> MPYSVGFREADAATSFLRAARSGNLDKALDHLRNGVDINTCNQNGLNGLHLASKEGHVKMVVELLHKEIILETTTKKGNTALHIAALAGQDEVVRELVNYGANVNAQSQKGFTPLYMAAQENHLEVVKFLLENGANQNVATEDGFTPLAVALQQGHENVVAHLINYGTKGKVRLPALHIAARNDDTRTAAVLLQNDPNPDV;> MSSKYPRSVRRCLPLWALTLEAALILLFYFFTHYDASLEDQKGLVASYQVGQDLTVMAALGLGFLTSNFRRHSWSSVAFNLFMLALGVQWAILLDGFLSQFPPGKVVITLFSIRLATMSAMSVLISAGAVLGKVNLAQLVVMVLVEVTALGTLRMVISNIFNTDYHMNLRHFYVFAAYFGLTVAWCLPKPLPKGTEDNDQRATIPSLSAMLGALFLWMFWPSVNSPLLRSPIQRKNAMFNTYYALAVSVVTAISGSSLAHPQRKISMTYVHSAVLAGGVAVGTSCHLIPSPWLAMVLGLVAGLISIGGAKCLPVCCNRVLGIHHISVMHSIFSLLGLLGEITYIVLLVLHTVWNGNGMIGFQVLLSIGELSLAIVIALTSGLLTGLLLNLKIWKAPHVAKYFDDQVFWKFPHLAVGF;>[2x]MRFTFPLMAIVLEIAMIVLFGLFVEYETDQTVLEQLNITKPTDMGIFFELYPLFQDVHVMIFVGFGFLMTFLKKYGFSSVGINLLVAALGLQWGTIVQGILQSQGQKFNIGIKNMINADFSAATVLISFGAVLGKTSPTQMLIMTILEIVFFAHNEYLVSEIFKASDIGASMTIHAFGAYFGLAVAGILYRSGLRKGHENEESAYYSDLFAMIGTLFLWMFWPSFNSAIAEPGDKQCRAIVNTYFSLAACVLTAFAFSSLVEHRGKLNMVHIQNATLAGGVAVGTCADMAIHPFGSMIIGSIAGMVSVLGYKFLTPLFTTKLRIHDTCGVHNLHGLPGVVGGLAGIVAVAMGASNTSMAMQAAALGSSIGTAVVGGLMTGLILKLPLW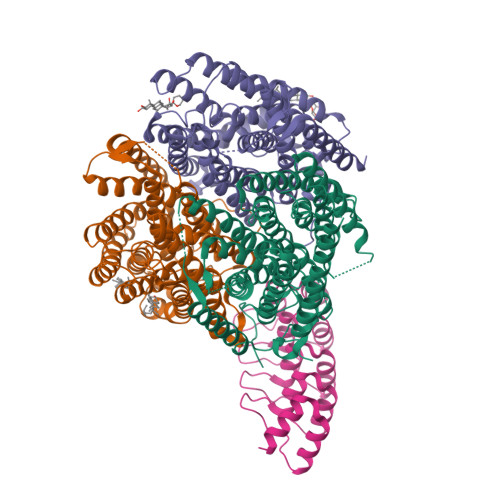GQPSDQNCYDDSVYWKVPKTR> AAL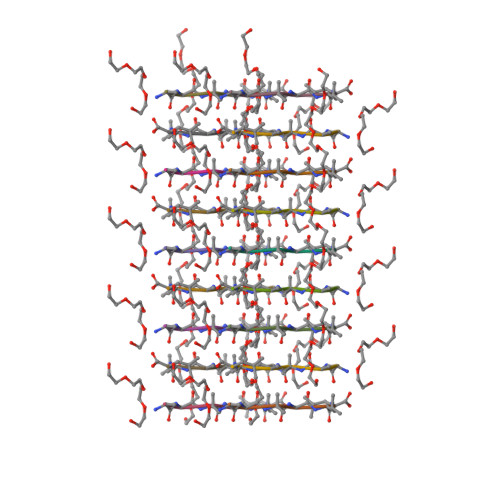ALL>[4x]MTASVSNTQNKLNELLDAIRQEFLQVSQEANTYRLQNQKDY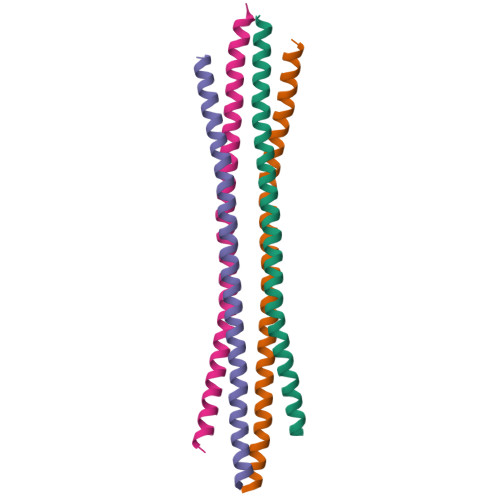DFKMNQQLAEMQQIRNTVYELELTHRKMKDAYEEEIKHLKLGLEQRDHQIA>[2x]MGFSDLRDKVVIVTGASMGIGRAIAERFVDEG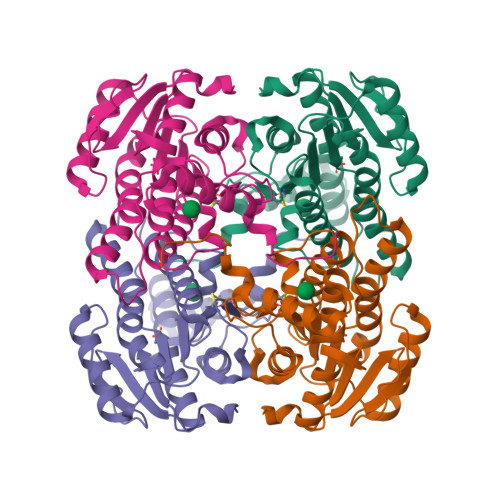SKVIDLSIHDPGEAKYDHIECDVTNPDQVKASIDHIFKEYGSISVLVNNAGIESYGKIESMSMGEWRRIIDVNLFGYYYASKFAIPYMIRSRDPSIVNISSVQASIITKNASAYVTSKHAVIGLTKSIALDYAPLLRCNAVCPATIDTPLVRKAAELEVGSDPMRIEKKISEWGHEHPMQRIGKPQEVASAVAFLASREASFITGTCLYVDGGLSIRAPISTPELEHHHHHH>[4x]MGMEMDKNLVREVIAKRVAQEFHDGYVVNLGIGLPTLVANYVGDMDVIFQSENGCIGVGPAPEKGKEDPYLVNAGAGFITAAKGAMFFDSAYSFGIIRGGHVDATVLGALEVDEKGNLANWMIPGKKVPGMGGAMDLVVGAKKVIVAME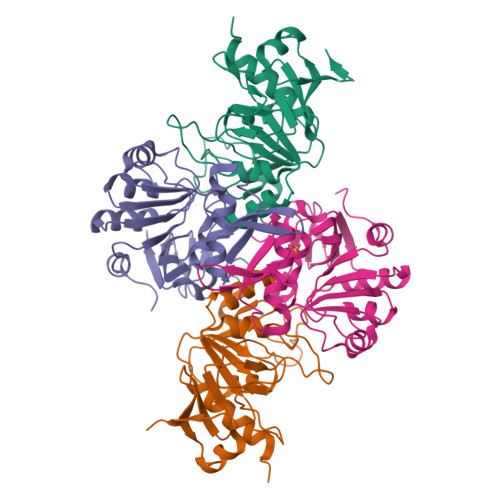HTSNGAIKILKECKLPLTAVGVVDLIITEKAVFEVTDKGLVLKEITPYSSLEDIKATTAADFIIADDLKK;>[4x]MGHHHHHHMKQKIVSMEEAISHVKDGMTVHIGGFIACGTPESIITALIEKGVKDLTIVANDTGLIDKGIGRLVVNNQVKKVIASHIGTNPETGRRMQSGEMEVELVPQGTLAERVRAAGYGLGGILTPTGLGTIVQEGKQIINVDGKDYLLEKPIKADVALIFGTKVDELGNVICEKTTKNFNPLMATAADVVIVEALEIVPAGSLSPEHLDISRIFIDYIVKSK>[6x]MEQYSEACIEACIDCMKACNHCFTKCLEESVQHHLSGCIRLDRECADICALAVKAMQTDSPFMKEICALCADICEACGTECGKHDHDHCQACAKACFTCAEQCRSMAA

The Csp3s are the cytosolic members of a new family of copper storage proteins. Both the M. trichosporium OB3b and B. subtilis proteins form tetramers of four-helix bundles possessing many Cys residues pointing into their cores, and can accommodate up to approximately 80 Cu(I) ions per tetramer. The number of Cu(I) ions a Csp can bind is dictated by how many Cys residues it possesses, with 18 and 19 respectively per monomer in MtCsp3 and BsCsp3 compared to 13 in MtCsp1. The Csp3s can bind copper in the cytosol of bacteria conferring the ability to grow at elevated levels of this metal.

A cytosolic Csp3 is also present in Bacillus subtilis, whose metal ion homeostasis has been studied in detail. The 18 Cys residues, all originating from α-helices, point into the core of the four-helix bundle of an apo-MtCsp3 monomer and none are involved in disulfide bonds, consistent with the Bradford:DTNB ratio data above. The crystal structure of apo-BsCsp3 has also been determined and the protein is a four-helix bundle like that of apo-MtCsp3 (the α-helical content in the structure is ~81%, very similar to the value of 83.1 ± 2.5% (n = 3) obtained from far-UV CD measurements, Supplementary Fig. S5). Apo-BsCsp3 also forms a tetramer, but αN is missing and consequently the apparent molecular weight in solution (46.0 ± 1.8 kDa, n = 8) matches that expected (47.4 kDa). The 19 Cys residues, also all from α-helices, point into the core of the bundle of apo-BsCsp3, with evidence of partial disulfide bond formation only between Cys38 and Cys81 in the crystal. In both Csp3 structures three highly conserved His residues are found at the more solvent exposed end of the four helix bundle. His104, His108 and His110 (His104 and His110 are ligands) from the α3-loop-α4 region are found around the opening to the bundle in MtCsp3 and are highly conserved among Csp3s, corresponding to His84, His86 and His88 in BsCsp3. Leu51 of MtCsp3, which is conserved in BsCsp3 (Leu35), corresponds to Met48 in MtCsp1 and its hydrophobic side chain appears to partially block the entrance (a Met is actually found in this position in a number of Csp3s). Copper coordination in MtCsp3 largely involves sites with two Cys ligands, with the most novel being Cu13, which as well as having two coordinating thiolates is bound by the side chain amide oxygen of Asn58. This Asn is not highly conserved in Csp3s, and an Asp is more common, as found in BsCsp3. Treatment with DTT has no significant effect on thiol quantification demonstrating that the Cys residues of both apo-Csp3s are not readily susceptible to oxidation. The Cys residues all originate from α-helices and the four-helix bundle scaffold provides the rigidity required to hold these residues sufficiently far apart to prevent thiol groups coupling via oxidation (in a cell this will be assisted by the reducing environment of the cytosol).> MHRVMGIETEYGISVPHQPNANAMAASSQVVNAYAPIGAPAQRQARWDFEEENPLRDARGFEVAREAADPSQLTDEDLGLANVILTNGARLYVDHAHPEYSTPEVTNPRDAVLWDKAGERIMAEAARRAADLPMGWTIQLYKNNTDNKGASYGCHENYLMNRSTPFADIVRHLIPFFVTRQVFCGAGRVGIGADGRGEGFQLSQRADFFEVEVGLETTLKRPIINTRDEPHADPEKYRRLHVIIGDANMSEIATYLKLGTTALVLAMIEDGFLSQDFSVESPVGALRAVSHDPTLRYQLRLHDGRRLTAVQLQMEYLEQARKYVEDRFGTDVDDMTRDVLDRWETTLVRLADDPMQLSRDLDWVAKLSILEGYRQRENLPWSAHKLQLVDLQYHDVRPDRGLYNRLVARGRMNLLVDEAAVRTAMHEPPNDTRAYFRGRCLAKFGAEIAAASWDSVIFDLPGRDSLQRVPTLEPLRGTRAHVGDLLDRCRSATELVAALTGGENLYFQ;> DAILDEIDDVLEENAEEFVRSYIQKGGE

Pupylation is the post-translational modification of lysine side chains with prokaryotic ubiquitin-like protein (Pup) that targets proteins for proteasomal degradation in mycobacteria and other members of Actinobacteria. A single Pup ligase enzyme, PafA (proteasome accessory factor A), is responsible for modifying all pupylation substrate proteins and likewise a single depupylase enzyme, Dop (deamidase of Pup), removes Pup from Pup-protein adducts. Depupylase Dop is structurally homologous to Pup ligase PafA, although the two evolutionarily related enzymes catalyze opposing reactions. Rather, before the catalytic cycle of Dop can begin, Dop-mediated cleavage of ATP in the active site must take place to generate the Pi species important for catalysis.

The phosphorylated Pup intermediate resulting from phosphoryl transfer to the amide side-chain of the C-terminal residue should only exist transiently in solution and be readily hydrolyzed after its formation. However, when crystals of Dop-PupE complex were soaked with ATP for 19 h, we serendipitously produced Dop with a bound phosphorylated Pup fragment and ADP in the active site. Presumably due to the high concentration of KH2PO4 in the crystallization solution, a potassium (K+) ion instead of a Mg2+ ion was identified at the n2 site, as indicated by the strong anomalous signal peak from data collected at around 2.0 Å wavelength, although under physiological conditions the n2 site is most likely occupied by a Mg2+ ion. However, the binding of K+ at the n2 site does not affect the binding of ADP and the C-terminal Pup residue, as both bind in a similar conformation as observed in the transition state complex. The carbamidyl phosphate moiety produced in the active site of Dop through a transition state of phosphoryl transfer is stabilized through coordination with three Mg2+ ions bound at the n1, n2 and n3 sites. In the subsequent step, a nearby water molecule, most likely activated by the side chain of D94, is responsible for hydrolysis of the glutaminyl-phosphate intermediate. With the crystal structures of Dop-Pup complexes in all intermediate states of ATP hydrolysis in hand, including the ground state (Dop-PupQ-AMP-PCP), the transition state of phosphoryl transfer (Dop-PupE-ADP-MgF3(H2O)−), the Pup-phosphorylated state (Dop-PupP-ADP) and the product state (Dop-PupE-ADP-MgF42−), we can develop a full mechanistic model for the generation of the catalytic Pi species.> MKSVKYISNMSKQEKGYRVYVNVVNEDTDKGFLFPSVPKEVIENDKIDELFNFEHHKPYVQ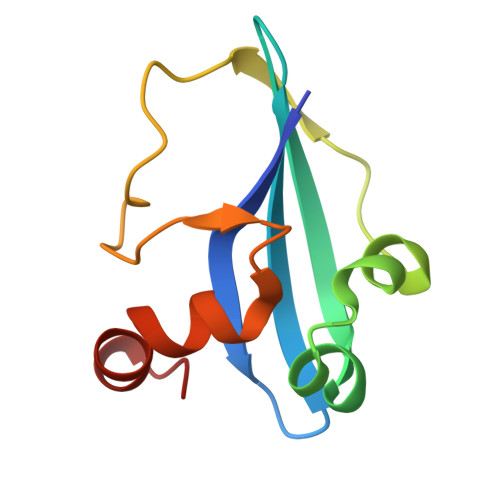KAKSRYDKNGIGYKIVQLDEGFQKFIELNKEKMKENLDY>[2x]KQGLTAGLAEAVRTSQPEHSVDAIRKAKKGLLDFTAASFAGREDKGIQKLLRLIEDEGGRPLVPIIGQGKKAAPLQSAMLNGFIAHALDFDDVHSDVRGHPSAVIVPALIASAARGHDERLLGAYIVGVEVMARLGESIGSRHYEKGWHNTGTLGAIAAACAVGYAEELTQEELEKAIGFAATQSAGMRVQFGTEMKPLHAGLAAQAGLLAVKLAQSEFGGSRTAFDGETGFFSLYGDVEKAQHT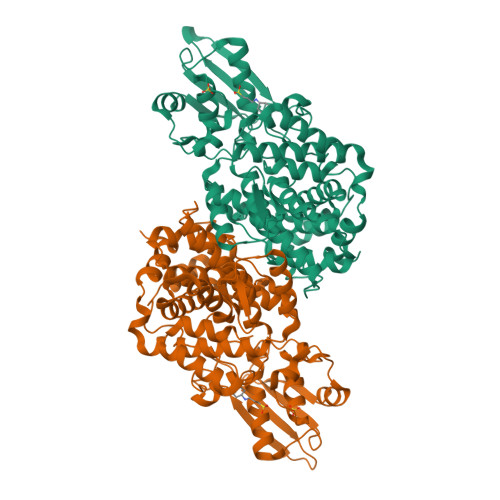LLNDWGAPWRIVQPGLWFKIYPFCSAAHHAADAVRQLISEETISAANTERIEVIFPPGGDAALTERSPKTGEEGRFSVEYVIALALHGHGLTVEHFSSQPIPNGIQTTIGHIQRVYDNATQPAPHAVPKGRFTIVRAYLSDGRICEARVDCPKGAPGNELSEEDIIEKLTLTVPQEKARRIITAVEKADIKEFLAHIELE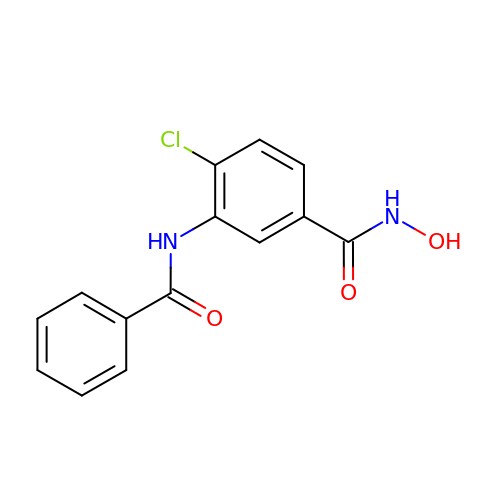3-benzamido-4-chloranyl-~{N}-oxidanyl-benzamide | C14 H11 Cl N2 O3 | BBBOKCZDRCMPOZ-UHFFFAOYSA-N> SMGKLSEQLKHCNGILKELLSKKHAAYAWPFYKPVDASALGVHDYHDIIKHPMDLSTVKRKMENRDYRDAQEFAADVRLMFSNC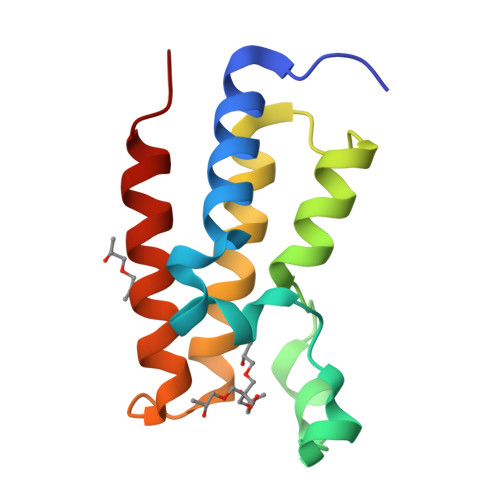YKYNPPDHDVVAMARKLQDVFEFRYAKMPD(2~{S})-2-(3-azanylpropyl)-5-[2,5-bis(fluoranyl)phenyl]-~{N}-methoxy-~{N}-methyl-2-phenyl-1,3,4-thiadiazole-3-carboxamide | C20 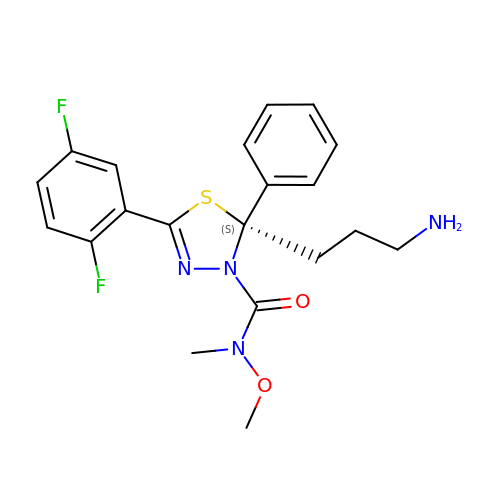H22 F2 N4 O2 S | LLXISKGBWFTGEI-FQEVSTJZSA-N> MALPLLASRRLFSSFVFRGQPSTLSSNLSLVRIRGLHGGSLSPPSATLPRAVQLFSSRIAFSTAAAEDSGASQTLEGRYASALFRVAKKKNQLEKVYGDLESVRNALKDSSEFRLFVDSPAVSVQQKLDVLRQLVNRYKFDPLTGNLLTTLVENKRLPMLAR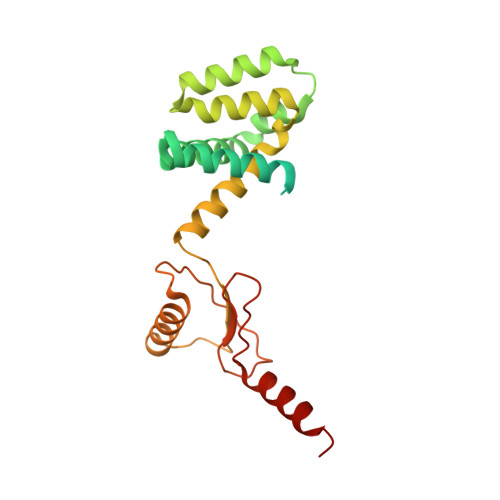VADAFDAMYRKEKGEVKCLVTSAKPLSAQQQKEIVAALQNRAGTQARLIIDYAVSPQIMGGLVVRLGEQVLDFSVATRLDRLQSQLLAPL> CGFGGSGSNGEGKKDSKGKTTLNINIKTEPFSLHPGLANDSVSGGVIRQTFEGLTRINADGEPEEGMASKIETSKDGKTYTFTIRDGVKWSNGDPVTAQDFEYAWKWALDPNNESQYAYQLYYIKGAEAANTGKGSLDDVAVKAVNDKTLKVELNNPTPYFTELTAFYTYMPINKKIAEKNKKWNTNAGDDYVSNGPFKMTAWKHSGSITLEKNDQYWDKDKVKLKKIDMVMINNNNTELKKFQAGELDWAGMPLGQLPTESLPTLKKDGSLHVEPIAGVYWYKFNTEAKPLDNVNIRKALTYSLDRQSIVKNVTQGEQIPAMAAVPPTMKGFEDNKEGYFKDNDVKT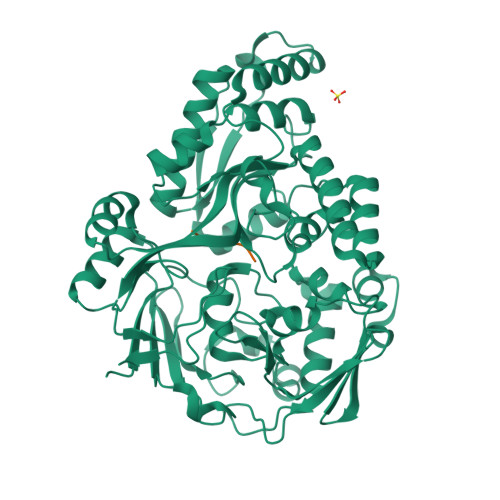AKEYLEKGLKEMGLSKASDLPKIKLSYNTDDAHAKIAQAVQEMWKKNLGVDVELDNSEWNVYIDKLHSQDYQIGRMGWLGDFNDPINFLELFRDKNGGNNDTGWENPEFKKLLNQSQTETDKTKRAELLKKAEGIFIDEMPVAPIYFYTDTWVQDENLKGVIMPGTGEVYFRNAYFK;> SRNVT>[2x]ESYLSPAQSVKPKINTEEKLPREKLNPPTPSIYLESKRDAFSPVLLQFCTDPRNPITVIRGLAGSLRLNLGLFSTKTLVEASGEHTVEVRTQVQQPSDENWDLTGTRQIWPCESSRSHTTIAKYAQYQASSFQESLQEELEVLFQGP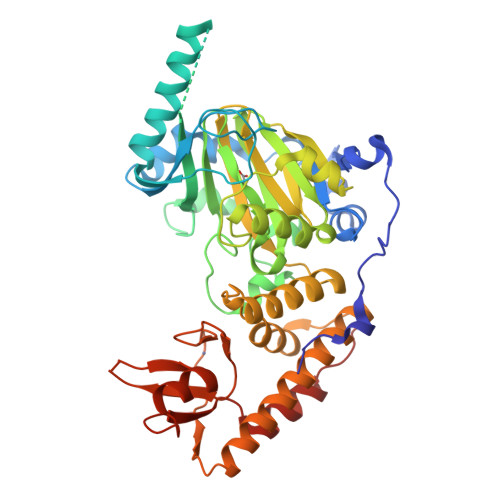TKAARKSAPATGGGSSGSHHIIKFGTNIDLSDAKRWKPQLQELLKLPAFMRVTSTGNMLSHVGHTILGMNTVQLYMKVPGSRTPGHQENNNFCSVNINIGPGDCEWFAVHEHYWETISAFCDRHGVDYLTGSWWPILDDLYASNIPVYRFVQRPGDLVWINAGTVHWVQATGWCNNIAWNVGPLTAYQYQLALERYEWNEVKNVKSIVPMIHVSWNVARTVKISDPDLFKMIKFCLLQSMKHCQVQRESLVRAGKKIAYQGRVKDEPAYYCNECDVEVFNILFVTSENGSRNTYLVHCEGCARRRSAGLQGVVVLEQYRTEELAQAYDAFTLAPASTSR>[3x]MGHHHHHHGQQDVHGPFQGQRQNEFDLMFVKEIFKNHNSNVVLSPFSVKILLTLIYEASDTSFGNAVSNTKRELSSVIQNDNIDHTRSYYKQLLESAQQDNKDYDLNIATNFFVDDFIEVINKYQQIANTHYHAMLEKVSYSNPTQTAATINNWVSEHTNGRL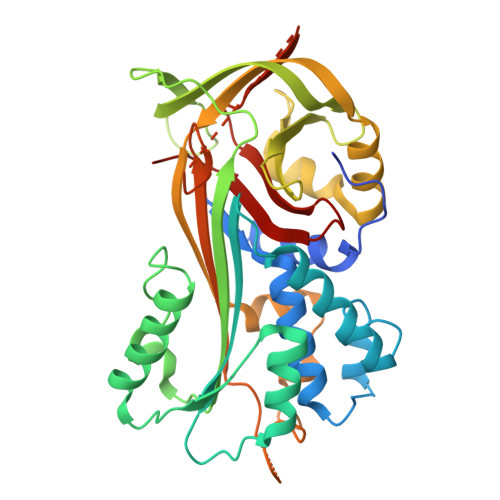REIVTPDSLEGAVITLVNVIYFCGLWTYPFPEVANNVKPFYGTRGKPTNAQYMEQNGQFYYDNSADLGAQILRLPYRGNKLAMYFILPNPDNTVNQVLDRINSASLHQALWYMEENEVNVTLPKFKFDFSEQLNEPLQQVGIREIFSQNASLPLLARGRGARDEVRVSRIFQKAGITINELGSEAYAATEIQLVNKFGGDGVQIFNANRPFIFFIEDETLGTMLFAGKIENPVF9-(2-DEOXY-5-O-PHOSPHONO-BETA-D-ERYTHRO-PENTOFURANOSYL)-6-(PHOSPHONOOXY)-9H-PURINE | C10 H14 N4 O10 P2 | 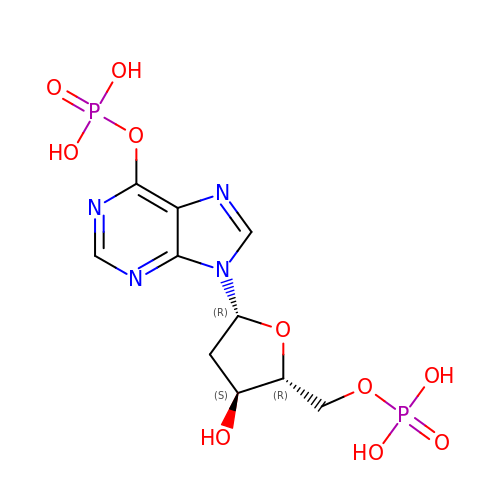GEECATYOCBMMIR-RRKCRQDMSA-N>SNARSSVAEQEADRDIIRFGEVSFSQLAEGVWMHTTYLDLMGFGPIPSNGLLVVNGDNTILVDTAWTDEQTEQIVAWASMVLAKPVRAAVVTHAHQDKMGGMAALHGANIATWAHPLSNELAPEEGLVPARNAITFDANGWATGEAAQSLAPLRLYYPGGAHTRDNITVGLPELGIAFGGCMIKAGDASNLGNLADADTAAYAQSVRNFAAAFPDART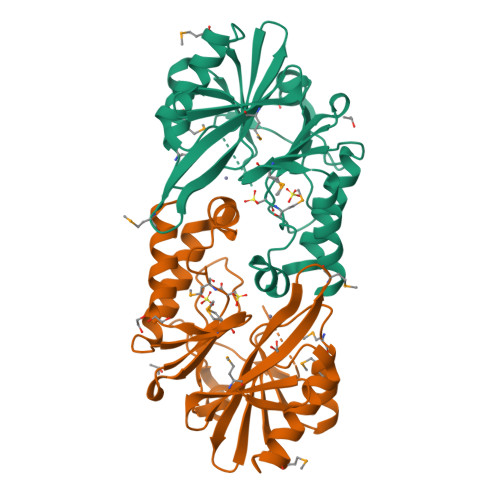IAMSHSPPEGRKAIERTLDLAEEL[2x]>[3x]SMDLSNKIKAAAEYIKGKSKYNPTIGLILGSGLGAIADQIEDAEYFPYNEIPNFPVSTVEGHAGRLVIGKFQGKEVVAMQGRFHYYEGYSMQEVTCPVRVMRLLGVETLVVTNAAGAVNKDYTPGDLMIISDHLNLSGSNPLIGKNLNEFGTRFPDMSNAYDKDLRAQVKDIAKNLGIEVREGV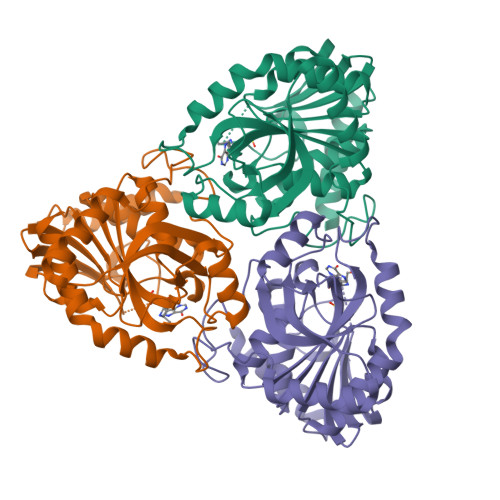YAMFSGPTYETPAEVRMARILGADAVGMSTVPEVIIANHSGMKVIGVSCMTNMAAGILEQPLNHEEVMETSAKVRKTFIELMTNIIKEI> MSKAGKKVKAQQHGHLADHVSVGETQIPKASTQHLLRKAGSLSAAGDTEVPIRGFVHMKLHKLVQKSLLAMQLAKRKTIMKSDVKKAAEL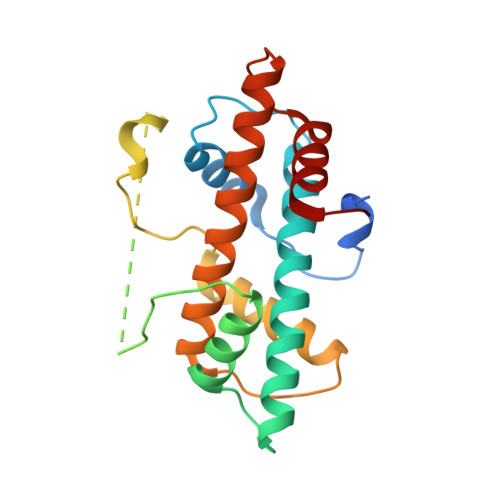MHLPVFAIPTKDSGAKGSVFLSCRQKGAGSAGTGSETNSQEVRSQMKSTCLIIPKERFRTMAKEISKKEGHDVHIAEAALDMLQVIVESCTVRLLEKALVITYSGKRTRVTSKDIETAFMLEHGPL> MHHHHHHMPSPNLPPGFDFTDPAIYAERLPVAEFAELRSAAPIWWNGQDPGKGGGFHDGGFWAITKLNDVKEISRHSDVFSSYENGVIPRFKNDIAREDIEVQRFVMLNMDAPHHTRLRKIISRGFTPRAVGRLHDELQERAQKIAAEAAAAGSGDFVEQVSCELPLQAIAGLLGVPQEDRGKLFHWSNEMTGNEDPEYAHIDPKASSAELIGYAMKMAEEKAKNPADDIVTQLIQADIDGEKLSDDEFGFFVVMLAVAGNETTRNSITQGMMAFAEHPDQWELYKKVRPETAADEIVRWATPVTAFQRTALRDYELSGVQIKKGQRV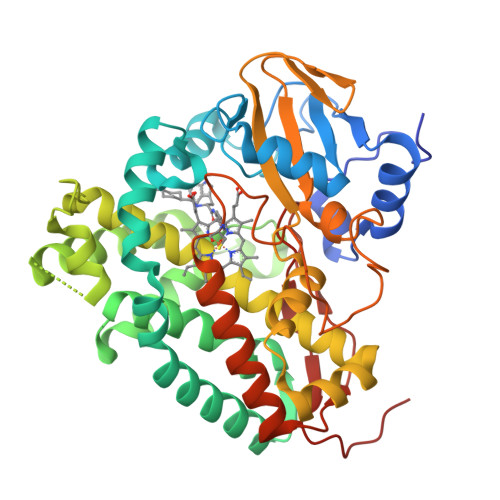VMFYRSANFDEEVFQDPFTFNILRNPNPHVGFGGTGAHYCIGANLARMTINLIFNAVADHMPDLKPISAPERLRSGWLNGIKHWQVDYTGRLPVAH(2S)-N-(4-cyano-3-iodophenyl)-3-(4-cyanophenoxy)-2-hydroxy-2-methylpropanamide | C18 H14 I N3 O3 | 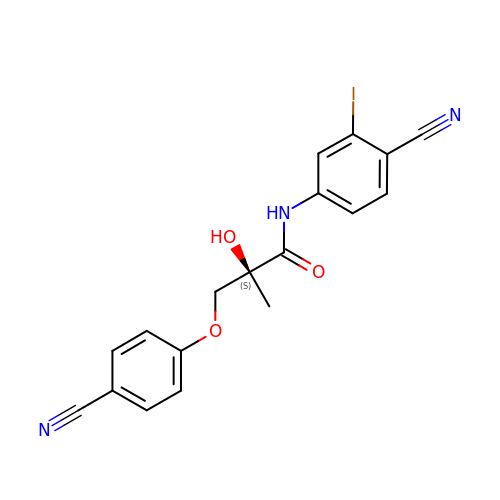RXSZCFAPSDTELY-SFHVURJKSA-N>[2x]ADPGAPAPVNPCCYYPCQHQGICVRFGLDRYQCDCTRTGYSGPNCTIPEIWTWLRTTLRPSPSFIHFLLTHGRWLWDFVNATFIRDTLMRLVLTVRSNLIPSPPTYNIAHDYISWESFSNVSYYTRILPSVPRDCPTPMGTKGKKQLPDAEFLSRRFLLRRKFIPDPQGTNLMFAFFAQHFTHQFFKTSGKMGPGFTKALGHGVDLGHIYGDNLERQYQLRLFKDGKLKYQMLNGEVYPPSVEEAPVLMHYPRGIPPQSQMAVGQEVFGLLPGLM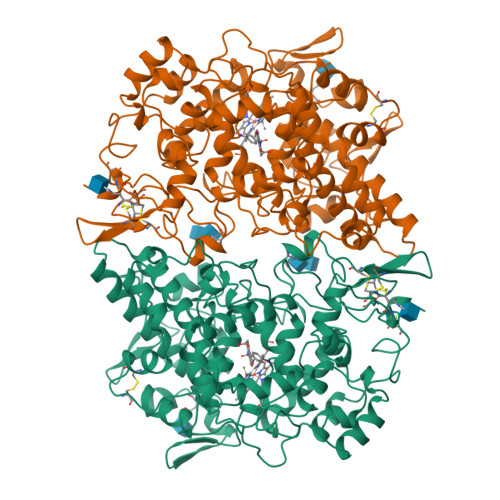LYATIWLREHNRVCDLLKAEHPTWGDEQLFQTARLILIGETIKIVIEEYVQQLSGYFLQLKFDPELLFGAQFQYRNRIAMEFNQLYHWHPLMPDSFRVGPQDYSYEQFLFNTSMLVDYGVEALVDAFSRQPAGRIGGGRNIDHHILHVAVDVIKESRVLRLQPFNEYRKRFGMKPYTSFQELTGEKEMAAELEELYGDIDALEFYPGLLLEKCHPNSIFGESMIEMGAPFSLKGLLGNPICSPEYWKASTFGGEVGFNLVKTATLKKLVCLNTKTCPYVSFHVPDPRQEDRPGVERPPTEL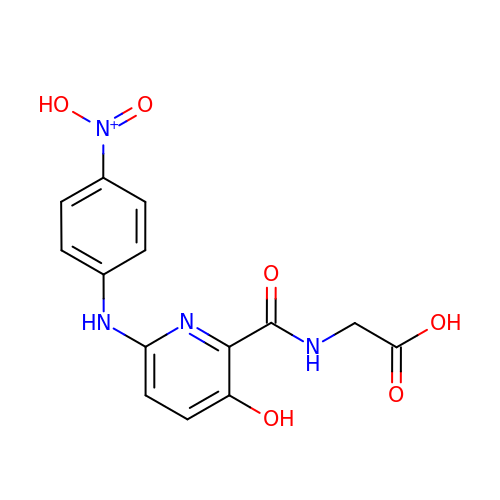2-[[6-[(4-nitrophenyl)amino]-3-oxidanyl-pyridin-2-yl]carbonylamino]ethanoic acid | C14 H13 N4 O6 | ISGBDWMUHZDQRG-UHFFFAOYSA-O> MIKSTDRKLVVGLEIGTAKVSALVGEILPDGMVNIIGVGNCPSRGMDKGGVNDLESVVKCVQRAIDQAELMADCQISSVYLALSGKHISCQNEIGMVPVSEEEVTQDDVDSVVHTAKSVRVRDEHRILHVIPQEYAIDYQEGIKNPVGLSGVRMQAKVHLITCHNDMAKNIVKAVERCGLKVDQLIFAGLAASYAVLTEDERELGVCVVDIGGGTMDVAVYTGGALRHTKVIPYAGNVVTSDIAYAFGTPPSDAETIKVRHGCALGSIVSKDESVEVPSVGGRPPRSLQRQTLAEVIEPRYTELLNLVNDEILRLQEQLRQQGVKHHLAAGIVLTGGGAQIDGLAECAQRVFHTQVRIGRPLNITGLTDYVQAPCYSTAVGLLHYGKESHLGGDSD

During bacterial cell division, filaments of tubulin-like FtsZ form the Z-ring, which is the cytoplasmic scaffold for divisome assembly. In Escherichia coli, actin homologue FtsA anchors the Z-ring to the membrane and recruits divisome components, including bitopic FtsN. In E. coli and many other bacteria, FtsA is the main membrane anchor for the cell division ring, the Z-ring, which initiates and organises division.

The EcFtsA1-405 and XpFtsA1-396 structures showed single protofilaments with a “loose” longitudinal contact between the IIA and IIB subdomains.> SNAMDHLHRKLRDHEAAMFQQGYLDDQFSQLQKLQDDTSPDFVIEVMTMFFDDSEKLLNNM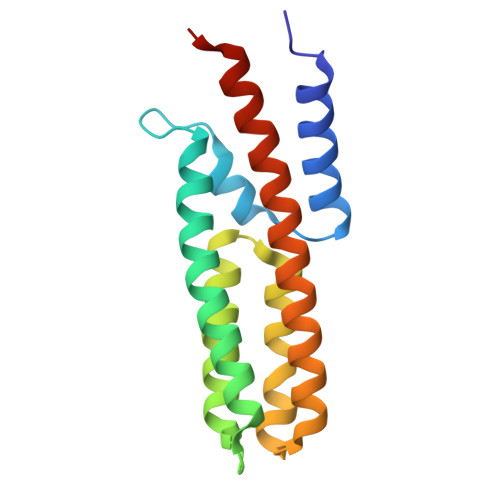SRALEQVPVNFKQIDAHAHQQKGSSASVGAARVKNVCGTFRNFCEAQNLEGCVRCLQQLQQEYSLLKNNLKYLFKLQQEIKTAGRSIHTRG>MPLSSQPAILIIGGAEDKVHGREILQTFWSRSGGNDAIIGIIPSASREPLLIGERYQTIFSDMGVKELKVLDIRDRAQGDDSGYRLFVEQCTGIFMTGGDQLRLCGLLADTPL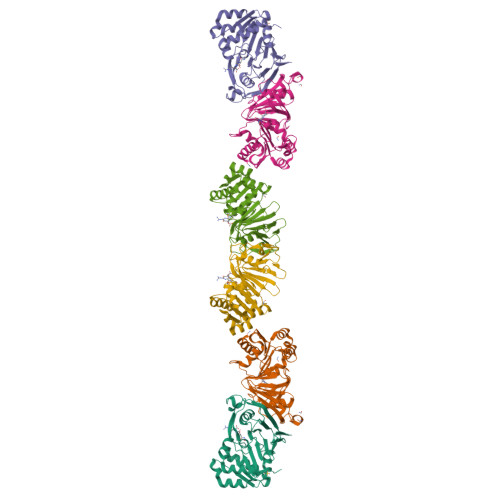MDRIRQRVHNGEISLAGTAAGAAVMGHHMIAGGSSGEWPNRALVDMAVGLGIVPEIVVDQHFHNRNRMARLLSAISTHPELLGLGIDEDTCAMFERDGSVKVIGQGTVSFVDARDMSYTNAALVGANAPLSLHNLRLNILVHGEVYHQVKQRAFPRVENLYFQ[3x]> AYTRYVDNNFCGPDGYPLECIKDLLARAGKASCTLSEQLDFIDTKRGVYCCREHEHEIAWYTERSEKSYELQTPFEIKLAKKFDTFNGECPNFVFPLNSIIKTIQPRVEKKKLDGFMGRIRSVYPVASPNECNQMCLSTLMKCDHCGETSWQTGDFVKATCEFCGTENLTKEGATTCGYLPQNAVVKIYCPACHNSEVGPEHSLAEYHNESGLKTILRKGGRTIAFGGCVFSYVGCHNKCAYWVPRASANIGCNHTGVVGEGSEGLNDNLLEILQKEKVNINIVGDFKLNEEIAIILASFSASTSAFVETVKGLDYKAFKQIVESCGNFKVTKGKAKKGAWNIGEQKSILSPLYAFASEAARVVRSIFSRTLETAQNSVRVLQKAAITILDGISQYSLRLIDAMMFTSDLATNNLVVMAYITGGVVQLTSQWLTNIFGTVYEKLKPVLD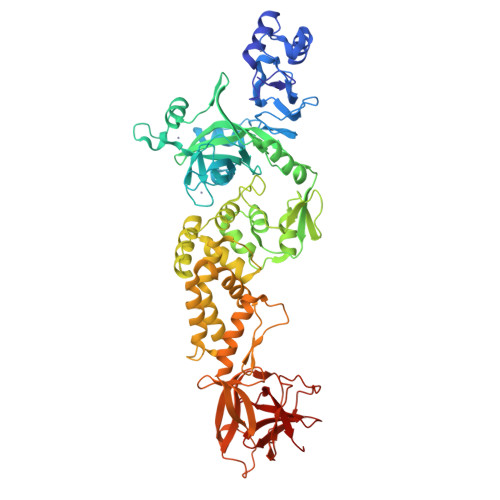WLEEKFKEGVEFLRDGWEIVKFISTCACEIVGGQIVTCAKEIKESVQTFFKLVNKFLALCADSIIIGGAKLKALNLGETFVTHSKGLYRKCVKSREETGLLMPLKAPKEIIFLEGETLPTEVLTEEVVLKTGDLQPLEQPTSEAVEAPLVGTPVCINGLMLLEIKDTEKYCALAPNMMVTNNTFTLKGG> MWYLLWFVGILLMCSLSTLVLVWLD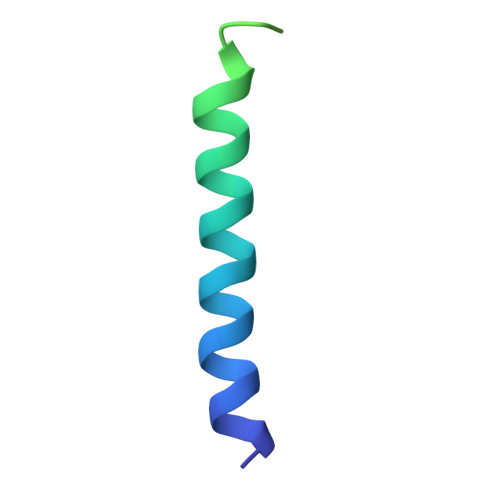PRLKSIEGRGTSGSSGSGSGGSGSGGGGWSHPQFEK> GSISIGIKCSPSIDLCEGQCRIRKYFTGY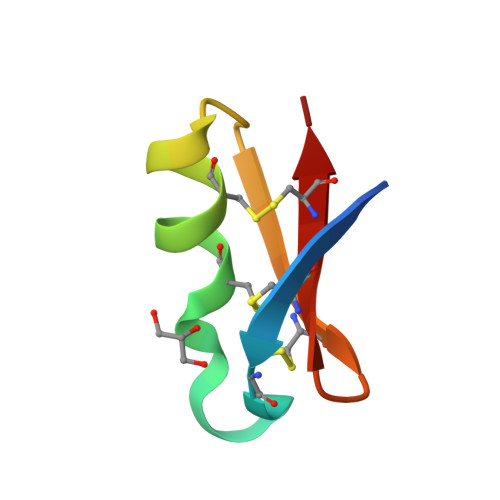CSGDTCHCSG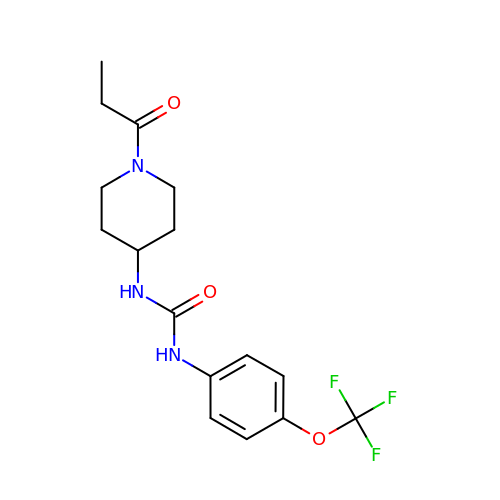1-(1-propanoylpiperidin-4-yl)-3-[4-(trifluoromethoxy)phenyl]urea | C16 H20 F3 N3 O3 | AAJMQTLFRTZCJK-UHFFFAOYSA-N>MLRSSNDVTQQGSRPKTKLGGSSMGIIRTCRLGPDQVKSMRAALDLFGREFGDVATYSQHQPDSDYLGNLLRSKTFIALAAFDQEAVVGALAAYVLPKFEQPRSEIYIYDLAVSGEHRRQGIATALINLLKHEANALGAYVIY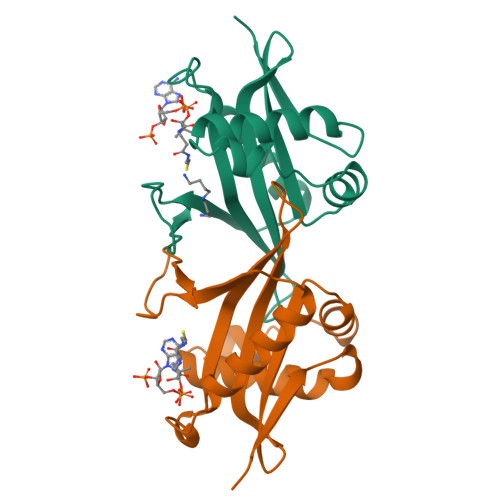VQADYGDDPAVALYTKLGIREEVMH[2x]>[2x]HHHHHHMTDK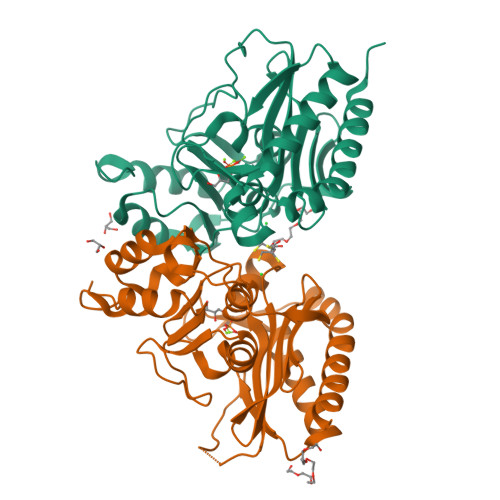TLQQIDKLICSWLKQIDNVIPQLIMEMTTETKRHRFDLVTNVDKQIQQQFQQFLATYFPEHQLLAEEKSNAMITNEINHLWIMDPIDGTANLVKQQEDYCIILAYFYEGKPMLSYVYDYPHKKLYKAIRGEGAFCNGIKMEEPPSLKLEDAIISFNAQVMNLDTVQDLFDASFSYRLVGACGLDSMRVAKGQFGAHINTNPKPWDIAAQFLFAELLNLKMTTLDGKAIDHLKGAPFIISNKACHETVLKILNANGGYQKYR Mutations in the LRRK2 gene, which encodes the leucine-rich repeat kinase 2 (LRRK2) protein, are among the most frequent genetic causes of late-onset PD and account for ~5% of familial and ~1% of sporadic cases. Most LRRK2-related PD mutations, such as G2019S (Gly2019→Ser), have increased kinase activity. Previous studies have suggested an emerging “Rab29–LRRK2–Rabs” cascade for LRRK2 signaling, in which GTP-bound Rab29 (Rab29•GTP) facilitates LRRK2 membrane recruitment and activation, then activated LRRK2 phosphorylates Rab GTPases, including Rab29 itself.

We determined cryo–electron microscopy (cryo-EM) structures of the Rab29–LRRK2 complex, reconstituted by mixing LRRK2, Rab29EM, GTP analog (GppNHp), adenosine triphosphate (ATP), and Mg2+. We thus introduced three point mutations (Q67L, T71A, and S72A) to Rab29 (Rab29EM) to maximize the opportunity of capturing the active Rab29•GTP–LRRK2 complex (where Q is glutamine, L is leucine, T is threonine, A is alanine, and S is serine). T71A and S72A prevent Rab29 phosphorylation, and Q67L abolishes GTPase activity and enhances the interaction between Rab29 and LRRK2 (26). The interaction conforms with a general Rab-effector recognition mode, in which effectors associate with the GTP-bound form of Rabs through the Switch I-Interswitch-Switch II surface. The surfaces of Rab29 and Rab10 predicted to interact with LRRK2 had almost identical interface residues, which is consistent with previous work suggesting that Rab10 interacts with LRRK2 at the Rab29 site. We also assessed the effect of interface mutations on LRRK2 kinase activity in cells by monitoring the phosphorylation status of Rab10-Thr73, Rab29-Thr71, and LRRK2-Ser1292 (28). All mutations introduced to the Rab29–LRRK2 interface had minor impacts on the basal activity of LRRK2 on Rab10 and Ser1292, supporting the view that the observed interface is important for LRRK2 recruitment but probably not for substrate recognition.

> MGSRDHLFKVLVVGDAAVGKTSLVQRYSQDSFSKHYKSTVGVDFALKVLQWSDYEIVRLQLWDIAGLERFAAMTRLYYRDASACVIMFDVTNATTFSNSQRWKQDLDSKLTLPNGEPVPCLLLANKCDLSPWAVSRDQIDRFSKENGFTGWTETSVKENKNINEAMRVLIEKMMRNS;> MASGSCQGCEEDEETLKKLIVRLNNVQEGKQIETLVQILEDLLVFTYSEHASKLFQGKNIHVPLLIVLDSYMRVASVQQVGWSLLCKLIEVCPGTMQSLMGPQDVGNDWEVLGVHQLILKMLTVHNASVNLSVIGLKTLDLLLTSGKITLLILDEESDIFMLIFDAMHSFPANDEVQKLGCKALHVLFERVSEEQLTEFVENKDYMILLSALTNFKDEEEIVLHVLHCLHSLAIPCNNVEVLMSGNVRCYNIVVEAMKAFPMSERIQEVSCCLLHRLTLGNFFNILVLNEVHEFVVKAVQQYPENAALQISALSCLALLTETIFLNQDLEEKNENQENDDEGEEDKLFWLEACYKALTWHRKNKHVQEAACWALNNLLMYQNSLHEKIGDEDGHFPAHREVMLSMLMHSSSKEVFQASANALSTLLEQNVNFRKILLSKGIHLNVLELMQKHIHSPEVAESGCKMLNHLFEGSNTSLDIMAAVVPKILTVMKRHETSLPVQLEALRAILHFIVPGMPEESREDTEFHHKLNMVKKQCFKNDIHKLVLAALNRFIGNPGIQKCGLKVISSIVHFPDALEMLSLEGAMDSVLHTLQMYPDDQEIQCLGLSLIGYLITKKNVFIGTGHLLAKILVSSLYRFKDVAEIQTKGFQTILAILKLSASFSKLLVHHSFDLVIFHQMSSNIMEQKDQQFLNLCCKCFAKVAMDDYLKNVMLERACDQNNSIMVECLLLLGADANQAKEGSSLICQVCEKESSPKLVELLLNSGSREQDVRKALTISIGKGDSQIISLLLRRLALDVANNSICLGGFCIGKVEPSWLGPLFPDKTSNLRKQTNIASTLARMVIRYQMKSAVEEGTASGSDGNFSEDVLSKFDEWTFIPDSSMDSVFAQSDDLDSEGSEGSFLVKKKSNSISVGEFYRDAVLQRCSPNLQRHSNSLGPIFDHEDLLKRKRKILSSDDSLRSSKLQSHMRHSDSISSLASEREYITSLDLSANELRDIDALSQKCCISVHLEHLEKLELHQNALTSFPQQLCETLKSLTHLDLHSNKFTSFPSYLLKMSCIANLDVSRNDIGPSVVLDPTVKCPTLKQFNLSYNQLSFVPENLTDVVEKLEQLILEGNKISGICSPLRLKELKILNLSKNHISSLSENFLEACPKVESFSARMNFLAAMPFLPPSMTILKLSQNKFSCIPEAILNLPHLRSLDMSSNDIQYLPGPAHWKSLNLRELLFSHNQISILDLSEKAYLWSRVEKLHLSHNKLKEIPPEIGCLENLTSLDVSYNLELRSFPNEMGKLSKIWDLPLDELHLNFDFKHIGCKAKDIIRFLQQRLKKAVPYNRMKLMIVGNTGSGKTTLLQQLMKTKKSDLGMQSATVGIDVKDWPIQIRDKRKRDLVLNVWDFAGREEFYSTHPHFMTQRALYLAVYDLSKGQAEVDAMKPWLFNIKARASSSPVILVGTHLDVSDEKQRKACMSKITKELLNKRGFPAIRDYHFVNATEESDALAKLRKTIINESLNFKIRDQLVVGQLIPDCYVELEKIILSERKNVPIEFPVIDRKRLLQLVRENQLQLDENELPHAVHFLNESGVLLHFQDPALQLSDLYFVEPKWLCKIMAQILTVKVEGCPKHPKGIISRRDVEKFLSKKRKFPKNYMTQYFKLLEKFQIALPIGEEYLLVPSSLSDHRPVIELPHCENSEIIIRLYEMPYFPMGFWSRLINRLLEISPYMLSGRERALRPNRMYWRQGIYLNWSPEAYCLVGSEVLDNHPESFLKITVPSCRKGCILLGQVVDHIDSLMEEWFPGLLEIDICGEGETLLKKWALYSFNDGEEHQKILLDDLMKKAEEGDLLVNPDQPRLTIPISQIAPDLILADLPRNIMLNNDELEFEQAPEFLLGDGSFGSVYRAAYEGEEVAVKIFNKHTSLRLLRQELVVLCHLHHPSLISLLAAGIRPRMLVMELASKGSLDRLLQQDKASLTRTLQHRIALHVADGLRYLHSAMIIYRDLKPHNVLLFTLYPNAAIIAKIADYGIAQYCCRMGIKTSEGTPGFRAPEVARGNVIYNQQADVYSFGLLLYDILTTGGRIVEGLKFPNEFDELEIQGKLPDPVKEYGCAPWPMVEKLIKQCLKENPQERPTSAQVFDILNSAELVCLTRRILLPKNVIVECMVATHHNSRNASIWLGCGHTDRGQLSFLDLNTEGYTSEEVADSRILCLALVHLPVEKESWIVSGTQSGTLLVINTEDGKKRHTLEKMTDSVTCLYCNSFSKQSKQKNFLLVGTADGKLAIFEDKTVKLKGAAPLKILNIGNVSTPLMCLSESTNSTERNVMWGGCGTKIFSFSNDFTIQKLIETRTSQLFSYAAFSDSNIITVVVDTALYIAKQNSPVVEVWDKKTEKLCGLIDCVHFLREVTVKENKESKHKMSYSGRVKTLCLQKNTALWIGTGGGHILLLDLSTRRLIRVIYNFCNSVRVMMTAQLGSLKNVMLVLGYNRKNTEGTQKQKEIQSCLTVWDINLPHEVQNLEKHIEVRKELAEKMRRTSVE> Y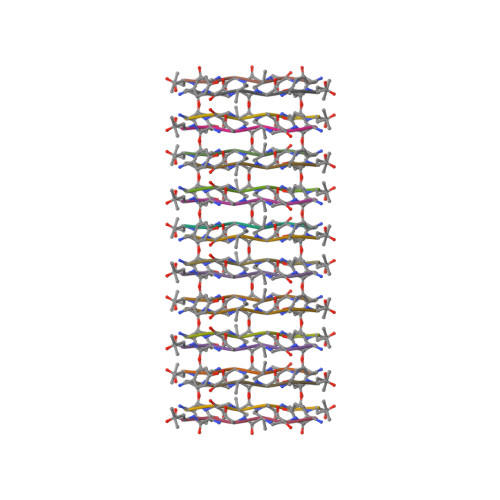TIAAL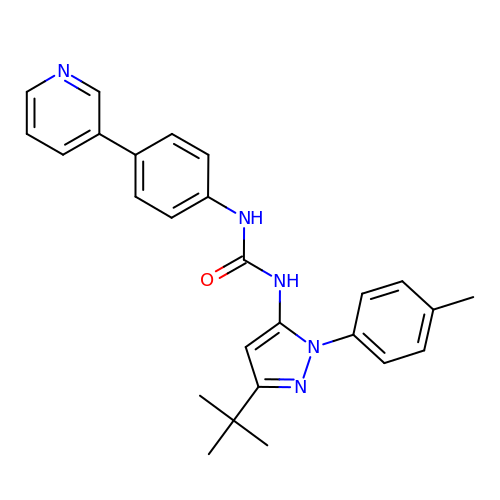1-[3-tert-butyl-1-(4-methylphenyl)-1H-pyrazol-5-yl]-3-[4-(pyridin-3-yl)phenyl]urea | C26 H27 N5 O | JMQOIKOCLOMDPW-UHFFFAOYSA-N>[6x]GSPASGTSLSAAIHRTQLWFHGRISREESQRLIGQQGLVDGLFLVRESQRNPQGFVLSLCHLQKVKHYLILPSEEEGRLYFSMDDGQTRFTDLLQLVEFHQLNRGILPCLLRHCCTRVAL;>[6x]SFEGYDNXC

Growth factor receptor-bound protein 7 (Grb7) is an adaptor protein involved in cell signaling where it interacts with a number of tyrosine kinases via its src-homology2 (SH2) domain78. In this way it plays a role in integrin dependant cell migration via its interaction with focal adhesion kinase and subsequent phosphorylation in focal contacts, consistent with its homology to the C. Elegans protein Mig-10 that is involved in cellular migration. It has been shown that overexpression of Grb7 enhances cell migration, while inhibition of Grb7 lowers the migratory potential of cells and is therefore linked with metastatic spread of cancer cells. While co-overexpression of Grb7 and ErbB2 occurs due to the proximity of their two genes on the 17q12-21 amplicon, Grb7 plays a role independent of ErbB2 in cancer progression. These important roles of Grb7 in numerous cancers have established Grb7 as a therapeutic target. Following the conventional nomenclature for SH2 domains, the Grb7-SH2 domain possesses a 3 stranded anti-parallel β-sheet consisting of the βB, βC and βD strands, flanked by 2 α-helices, αA and αB.

We show that the G7-B4 peptide binds with an improved binding affinity of KD = 0.83 μM and retains specificity for Grb7-SH2 domain over Grb2, Grb10 and Grb14-SH2 domains. In order to characterise the structural basis for the improved affinity of G7-B4 as compared to G7-B1 for Grb7-SH2 domain, we solved the structure of the Grb7-SH2/G7-B4 complex using X-ray crystallography to 2.47 Å resolution. The asymmetric unit consists of six Grb7-SH2 domains, six G7-B4 peptides, 75 water molecules, six malonic acid molecules and six formate molecules (present in the crystallisation conditions). The bound G7-B4 peptide is clearly defined in the electron density, and shows that the staple is again engaged in interactions with the Grb7-SH2 domain. The staple forms close contacts with Met495, Asp496, Asp497 backbone and sidechains in the EF loop of Grb7-SH2 and Ile 518 in the BG loop in the same way as seen for G7-B1. The staple contributes 55 Å2 of the total interaction surface area of 424 Å2. The G7-B4 structure, however, shows a loss of some close contacts that were present in G7-B1, including the loss of the salt bridges between E3 and Arg 462 in the BC loop, and the loss of a hydrogen bond between Y5(OH) and Ser460(OG). The Y5(OH) of G7-B4 also forms a hydrogen bond with a malonic acid that is bound in the Grb7-SH2 domain pY binding pocket, with the interaction occurring in a similar fashion to the phosphate interaction in the G7-B1 co-crystal structure. The thioether linkage is well defined in the electron density, positioned across the top of the stapled cyclic peptide, linking residues 1 and 8, but not altering their positions compared to those in the G7-B1 structure.> MNDHIHRVPALTEEEIDSVAIKTFERYALPSSSSVKRKGKGVTILWFRNDLRVLDNDALYKAWSSSDTILPVYCLDPRLFHTTHFFNFPKTGALRGGFLMECLVDLRKNLMKRGLNLLIRSGKPEEILPSLAKDFGARTVFAHKETCSEEVDVERLVNQGLKRVGNSTKLELIWGSTMYHKDDLPFDVFDLPDVYTQFRKSVEAKCSIRSSTR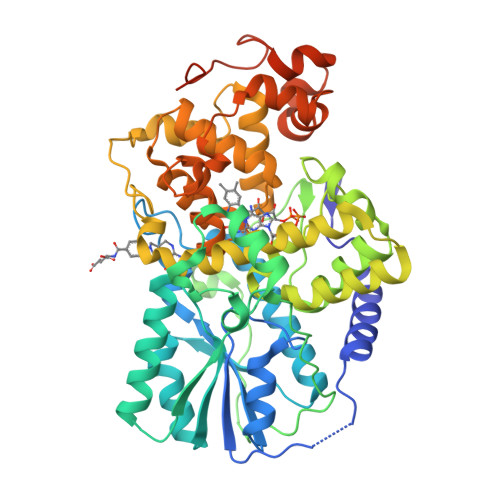IPLSLGPTPSVDDWGDVPTLEKLGVEPQEVTRGMRFVGGESAGVGRVFEYFWKKDLLKVYKETRNGMLGPDYSTKFSPWLAFGCISPRFIYEEVQRYEKERVANNSTYWVLFELIWRDYFRFLSIKCGNSLFHLGGPRNVQGKWSQDQKLFESWRDAKTGYPLIDANMKELSTTGFMSNRGRQIVCSFLVRDMGLDWRMGAEWFETCLLDYDPCSNYGNWTYGAGVGNDPREDRYFSIPKQAQNYDPEGEYVAFWLQQLRRLPKEKRHWPGRLMYMDTVVPLKHGNGPMAGGSKSGGGFRGSHSGRRSRHNGP> GCGXU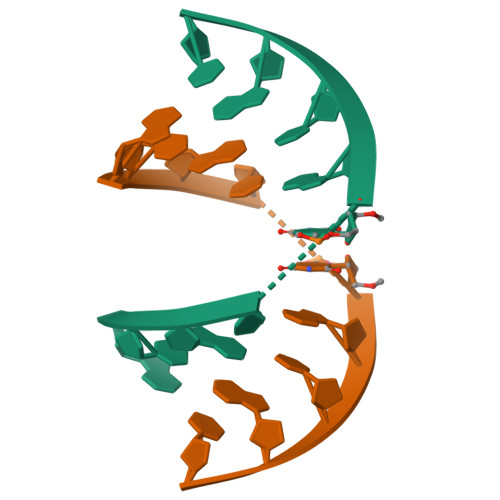ACGC>MASNFTQFVLVDNGGTGDVTVAPSNFANGVAEWISSNSRSQAYKVTCSVRQSSAQNRKYTIKVEVPKVATQ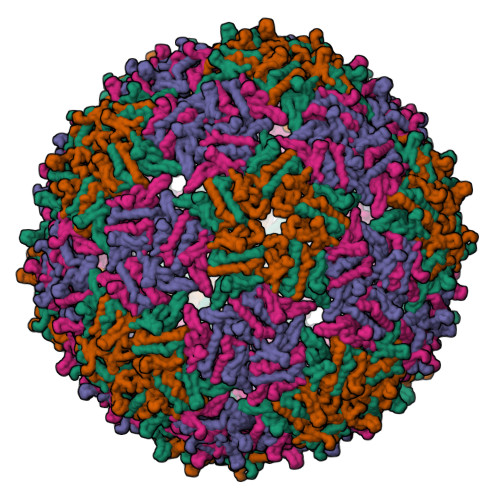TVGGVELPVAAWRSYLNMELTIPIFATNSDCELIVKAMQGLLKDGNPIPSAIAANSGIY[4x]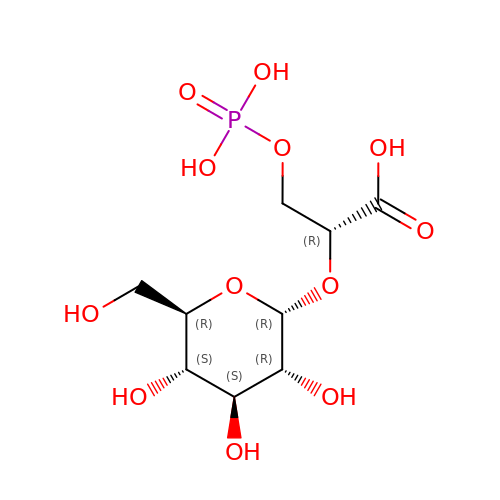(2R)-2-(alpha-D-glucopyranosyloxy)-3-(phosphonooxy)propanoic acid | C9 H17 O12 P | RJDBNSZFZDWPFL-CECBSOHTSA-N>[2x]MSSSKQYQQQPEDEELGPVTIAEDEVEEILDVEDPDGDVAMGSDDEGPEEIALENDSIAYFDGHKDSVFAIAQHPLYPNIVATGGSEGDADDAPGKGYVLDISAAAGRPVLPPSYNSDPSSAPQQNTSLNPIFEIDGHTDSINALTFTLPRGDFLVSGGMDGRMRVYAVSVPQNGALAQFKFLAESQETEEINWFAPCPSPDHPNTIALGASDGSVWVFTLDASDPSNPVQIVQSYFLHTGPCTAGAWSPDGLLLATVSEDESLHVYDVFGVAASKSLVTDNGQTVVSLTNVDQRFAVEGGLFSVAVSPTGAVVAVGGAGGQIKIVGLPRLSQPQQPQSQSQSRTGKAPAGRAGRPSQQQQTTSHQAGTILASLQIQSDNIESLAFSPSAPILAAGSTDGSIAVFDTSRSFALRRHLRGAHAEDPVVKVEFVKSPPNAAMAGWLLTSCGMDGVVRRWDLRGGTAGPGTLPHMQHLQQQRQQQQEGAAPSGLVKEWKGHRSGQEGGGVLGFVQGETGERIVTVGDDAVVLVFEAGSHHHHHH

In the case of Sqt1, we were able to decipher the mode of L10-N peptide binding by X-ray crystallography. These structural analyses showed that the C-terminal domain of Sqt1, which is preceded by a non-essential N-terminal extension of ∼50 amino acids, folds into an eight-bladed WD-repeat β-propeller. Moreover, the binding mode of the N-terminal residues of Rpl10 (L10-N) by the eight-bladed WD-repeat β-propeller of Sqt1, as revealed by X-ray crystallography, allows establishing a refined model for the final pre-60S maturation events that lead to the stable incorporation of Rpl10 and the release of Nmd3. Taken together, we propose that Sqt1 may protect Rpl10 from aggregation before and/or promote its incorporation into almost mature pre-60S subunits in the cytoplasm. We conclude that the β-propeller domains of Sqt1 and Rrb1, which harbour the essential function of these proteins, recognize the very N-terminal residues of Rpl10 and Rpl3.

To this end, we also performed in vitro binding assays with the orthologous proteins from the thermophilic, filamentous ascomycete Chaetomium thermophilum (ct), whose proteins often exhibit improved biochemical properties. Both ctSqt1 and ctSqt1.52C (deletion of amino acids 2–51), which fully complement the absence of Sqt1 in vivo, could be efficiently co-purified with ctRpl10 or its N-terminal 20 residues. As a first step towards the elucidation of the recognition mode of the N-terminal residues of Rpl10 by the predicted β-propeller domain of Sqt1 at the atomic level, we independently determined the crystal structure of ctSqt1 at 1.94 Å by molecular replacement and of ctSqt1.52C, lacking the dispensable N-terminal extension, at 1.5 Å resolution by single-anomalous dispersion (SAD) followed by molecular replacement using the ctSqt1.52C Se-Met structure as the search model. While the N-terminal extension could not be resolved, the crystal structures revealed that residues 52–533 of ctSqt1 form a typical eight-bladed WD-repeat β-propeller; thus, being composed of eight blades that each contain four β-strands and showing the characteristic ‘velcro' closure owing to the presence of the N-terminal β-strand as the outermost β-strand of the eighth blade. Sqt1 and ctSqt1 share a high degree of overall structural conservation and mainly differ in three ctSqt1-specific insertions located in the loops connecting β-strands 1c-1d, 5c-5d and 7c-7d. Analysis of the electrostatic properties revealed that both β-propeller structures notably contain a negatively charged top surface, whereas the bottom sides exhibit a charge-mixed surface.>[6x]MVEKFVGTWKIADSHNFGEYLKAIGAPKELSDGGDATTPTLYISQKDGDKMTVKIENGPPTFLDTQVKFKLGEEFDEFPSDRRKGVKSVVNLVGEKLV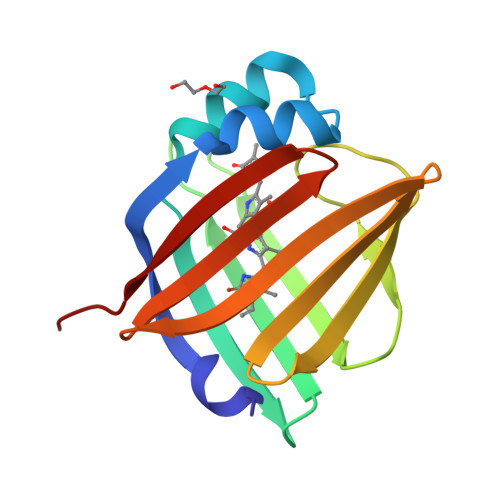YVQKWDGKETTYVREIKDGKLVVTLTMGDVVAVRSYRRATE> GSGGSGKVVKFSYMWTINNFSFCREEMGEVIKSSTFSSGANDKLKWCLRVNPKGLDEESKDYLSLYLLLVSCPKSEVRAKFKFSILNAKGEETKAMESQRAYRFVQGKDWGFKKFIRRDFLLDEANGLLPDDKLTLFCEVSVVQD;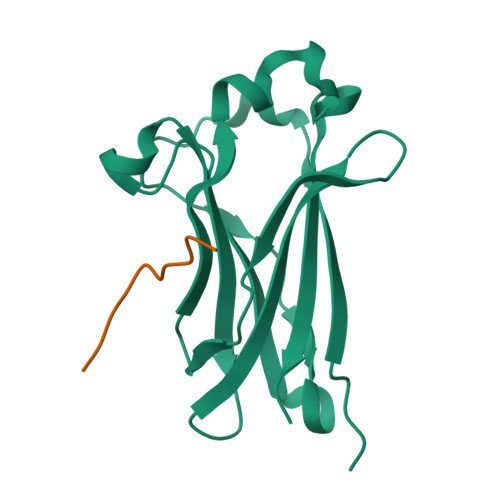> DEVTSTTSSS> RSPWGDELLNICMNAKHHKRVPSPEDKLYEECIPWKDNACCTLTTSWEAHLDVSPLYNFSLFHCGLLMPGCRKHFIQAICFYECSPNLGPWIQPVGSLGWEVAPSGQGERVVNVPLCQEDCEEWWEDCRMSYTCKSNW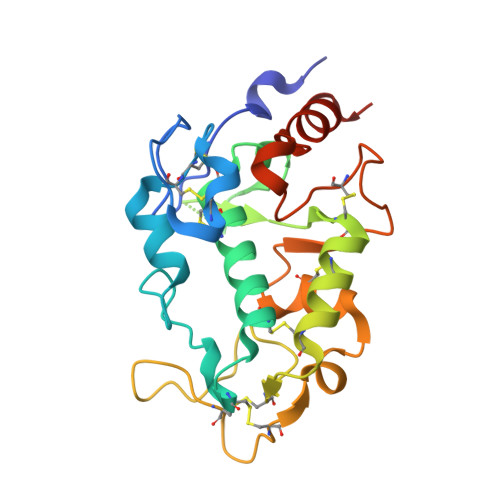RGGWDWSQGKNRCPKGAQCLPFSHYFPTPADLCEKTWSNSFKASPERRNSGRCLQKWFEPAQGNPNVAVARLFASEFLEVLFQ>APAPVPENGLEKRQSLSSVLSALSGLTEPTAILSQLEAVEATSTPTSVEQAQEQLEAIYGTTPTNIFENIAQQIADGLSTLTIVQALGFSPSGENSETNSNTREPSTTIYPKKSSSDAPYSITEEELRQAIYIPSDFTYGDKPPVIFVPGTGSYGGISFGSNLRKLLTGVSYADPVWLNVPDALLRDAQTNGEFVAYAINYISGISGDANVSVVSWSQGGLDTQWAFTYWPSTRALVSDFVPVSPDFHGTVLANVICLNPGAGGVGLGPCAPAVLQQEYNSNFVTALRAAGGADAYVPTTSVFSGFLDEIVQPQSGTGASAYINDARGVGTTNAEVQVVCKGKGPAGGFYTHESLLVNPLTYALLVDALTHDGPGSVDRLDLDTVCSTVVAPGLGLDALLEIEGVNVLAAVNLLTYSDRRLAEPALMSYAA[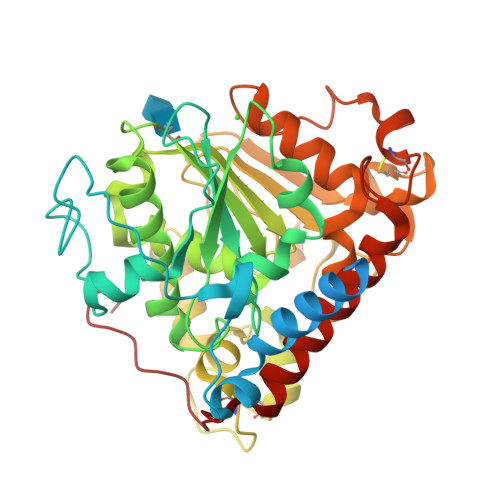2x]>AAGVAAWLPFARAAAIGWMPVASGPMPAPPRQERKRTQDALIVLNVSGTRFQTWQDTLERYPDTLLGSSERDFFYHPETQQYFFDRDPDIFRHILNFYRTGKLHYPRHECISAYDEELAFFGLIPEIIGDCCYEEYKDRRRENAERLQDDADTDTAGESALPTMTARQRVWRAFENPHTSTMALVFYYVTGFFIAVSVIANVVETVPCGSSPGHIKELPCGERYAVAFFCLDTACVMIFTVEYLLRLAAAPSRYRFVRSVMSIIDVVAILPYYIGLVMTDNEDVSGAFVTLRVFRVFRIFKFSRHSQGLRILGYTLKSCASELGFLLFSLTMAIIIFATVMFYAEKGSSASKFTSIPAAFWYTIVTMTTLGYGDMVPKTIAGKIFGSICSLSGVLVIALP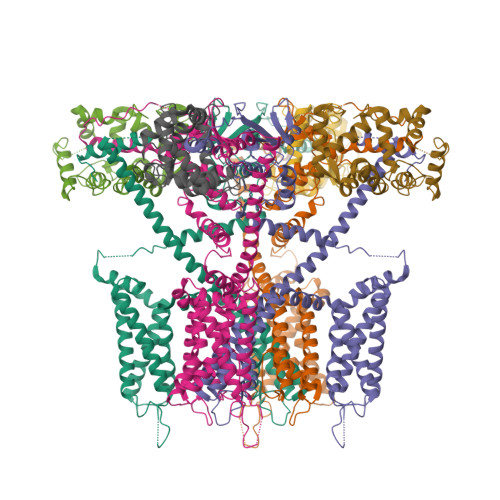VPVIVSNFSRIYHQNQRADKRRAQKKARLARIRAAKSGSANAYMQSKRSGLLSNQGRGDGSAFVTKSGSSFETQHHHLLHCLEKTTNHEFVD[4x];>PEGLEQLEAQTNFTKRELQVLYRGFKNECPSGVVNEDTFKQIYAQFFPHGDASTYAHYLFNAFDTTQTGSVKFEDFVTALSILLRGTVHEKLRWTFNLYDINKDGYINKEEMMDIVKAIYDMMGKYTYPVLKEDTPRQHVDVFFQKMDKNKDGIVTLDEFLESCQEDDNIMRSLQLFQNVM[4x]> GSTAEKNRKDAEEWFFTKTEELNREVATNSELVQSGKSEISELRRTMQNLEIELQSQLSMKASLENSLEETKGRYCMQLAQIQEMIGSVEEQLAQLRCEMEQQNQEY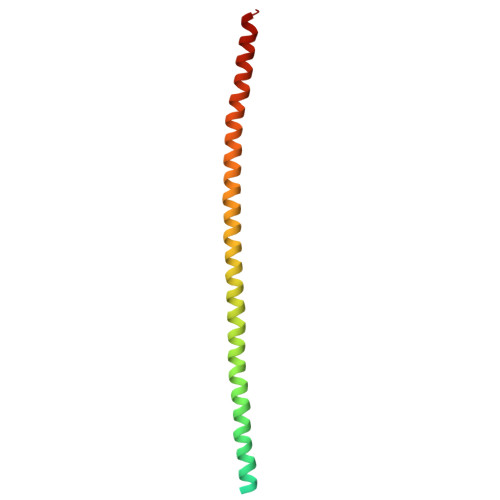KILLDVKTRLEQEIATYRRLLEGE>[4x]MHHHHHHSTPSIVIASAARTAVGSFNGAFANTPAHELGATVISAVLERAGVAAGEVNEVILGQVLPAGEGQNPARQAAMKAGVPQEATAWGMNQLCGSGLRAVALGMQQIATGDASIIVAGGMESMSMAPHCAHLRGGVKMGDFKMIDTMIKDGLTDAFYGYHMGTTAENVAKQWQLSRDEQDAFAVAS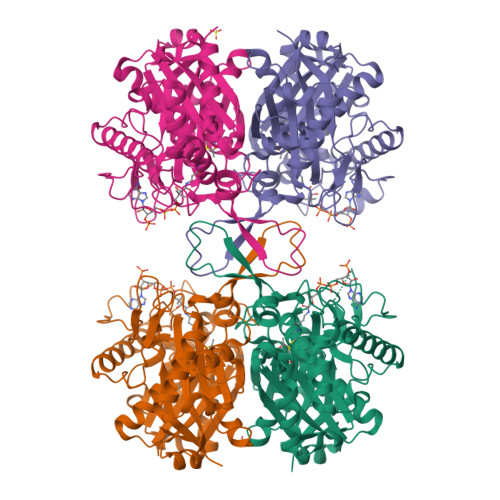QNKAEAAQKDGRFKDEIVPFIVKGRKGDITVDADEEIRHGATLDSMAKLRPAFDKEGTVTAGNASGLNDGAAAALLMSEAEASRRGIQPLGRIVSWATVGVDPKVMGTGPIPASRKALERAGWKIGDLDLVEANEAFAAQACAVNKDLGWDPSIVNVNGGAIAIGHPIGASGARILNTLLFEMKRRGARKGLATLCIGGGMGVAMCIESL> MIIANADGCTPYEVARGVTIVRGEGAYVYDAEGRGLIDLSNSFGSVMLGHQDPVVTEAVLKTVRSGVPAAASLDLQNHLAEQIAGDLPGDQRVAFFKTGTAATRAAASAARQVTGKRLIASCGYHGYDLMWEFTPPGQPNSEDVLHCYHLPELIDQVLDKHAHELAAVIIAPDYIHVSPEYIADLFERCERVGVVTIADEVKHGYRLRQGASVTEASVVADMYTYAKGISNGWPLSCVAGDERFLKPLAEFVSTLTFEAPSFAAASATLDRLAELDVQAQLAIDGARFVSEAAKMISTRDLPIEMAGTGAAFQFVCAEEVEEVLLPHALAEGLILEPSDQQYPSACFRGEVVDDALERLDRALTTMAAARPDLVGREVTQLDRVNAAFCQMDGLPGRPDGWSLDQCVEYVTAQL

GenB2 acts as an isomerase, converting C2a into C2 by changing the stereochemistry of the chiral center C-6′. Four genes encoding PLP-dependent enzymes (GenB1–GenB4) identified in the gentamicin BGC and a methyltransferase, GenL, from outside the BGC, are responsible for the last steps of gentamicin C complex biosynthesis. The structure of GenB2 shows, as expected, a characteristic PLP-dependent enzyme class I fold. Similar to other enzymes from this family, the active site of GenB2 is located in a deep cavity formed by a groove in the interface between the two protomers of the dimer, and each subunit contributes with essential residues for the substrate and cofactor binding.

In order to gather insights into the binding mode of GenB2 substrate gentamicin C2a, we have obtained the structure of GenB2 in complex with gentamicin G418 and gentamicin X2. G418 is produced from gentamicin X2 in earlier steps of gentamicin biosynthesis through methylation at C-6′ by GenK. G418 binds to a groove in GenB2, which is negatively charged and agrees with the complementary charge of a positively charged substrate. Also, several aromatic residues have face-to-face interactions with the sugar rings of the substrate. Thus, Tyr124 interacts with ring I, while Phe133 interacts with ring III. The ring I interacts via hydrogen bonds with Cys9 and Asp392. As expected, ring II, which is most deeply buried in the GenB2 structure, engages in a large number of direct and indirect interactions. It is possible to observe direct interactions with Lys227, Tyr342, Asp339, Lys202, Cys389, Gln390, and Asp392 and indirect interactions mediated by water molecules with Ser338, Gln340, Gln390, and Lys202. Interestingly, Cys9 in the complex of holo GenB2 with G418 adopts a double conformation in our structure in order to interact with the substrate. Our ligand-bound crystal structures show that the thiol of Cys9 in conformation 1 can hydrogen bond to the C-6′ amino group of gentamicin C2a and could, in its deprotonated form, be the base that deprotonates this initially protonated amine, allowing it to nucleophilically attack the internal aldimine.> UCCCAGUCCACCG;> CGGUGAGAAGGGXGGCAGAGAAACACAC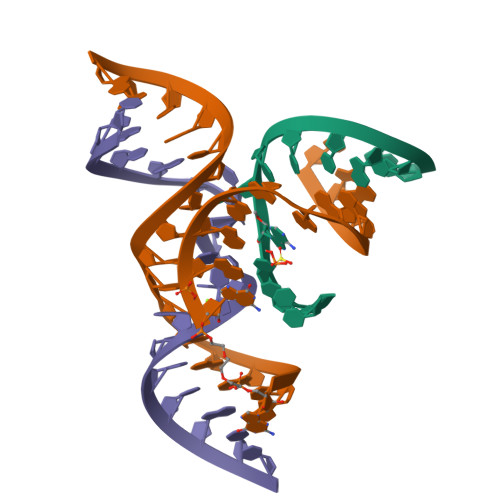GA;> UCGUGGUCCAUUACCUGCC Among them, Oligoribonuclease (Orn) is unique as its activity is required for clearing short RNA fragments, which is important for cellular fitness. Here, we show that Orn exhibits exquisite substrate preference for diribonucleotides. While other cellular RNases process oligoribonucleotides down to diribonucleotide entities, Orn is the one and only diribonucleotidase that completes the terminal step of RNA degradation. From this we propose a general model of RNA degradation, wherein a combination of exoribonucleases process oligoribonucleotides down to diribonucleotides and Orn completes RNA recycling by cleaving diribonucleotides to nucleoside monophosphates.

We initially determined the crystal structure of P. aeruginosa Orn (OrnPa) with diribonucleotide substrate; however, crystal packing contacts prevented substrate binding (data not shown). Instead, we were able to crystallize two representative homologs, OrnVc and the human REXO2 (also known as small fragment nuclease or Sfn [Bruni et al., 2013]), bound to the diribonucleotide pGpG (Figure 2—source data 1). Superimposing the two structures indicates their identical fold (rmsd of 0.75 Å for the protomer), which is preserved in the substrate-free Orn structure determined previously (rmsd of 0.54 Å for the protomer). The pGpG-bound structures reveal a narrow active site that is lined by the conserved acidic residues of the signature DEDD motif (D12, E14, and D112 of OrnVc; D15, E17, and D115 of REXO2) and the general base H158 or H162 in OrnVc or REXO2, respectively (Figure 2A and B and Figure 2—figure supplement 1B and Figure 2—source data 2). In OrnVc, the bases of the diribonucleotide buttress against aromatic residues W61 and Y129, the latter being contributed from the second half-side of the dimeric enzyme. Residue L18 in OrnVc (L21 in REXO2) wedges in-between the two bases. Most notably, residues S108, R130, S135 and the hydroxyl group on Y129 (S111, R133, S138, and Y132 in REXO2) form hydrogen bonds with the 5' phosphate of pGpG, capping the substrate. This phosphate cap creates a major constriction of the active site, which is not observed in structurally related 3'−5' exoribonucleases such as RNase T or ExoI (Figure 2C and Figure 2—figure supplement 1 and Figure 2—source data 2). By this assay, quantification of the diffusion zone reveals that OrnVc exhibits the highest affinity for diribonucleotide (Kd pGpG = 90 -/+9 nM), as compared to oligoribonucleotides of greater lengths. Mutations of the central phosphate cap residue R130 to alanine led to complete loss of catalytic activity, comparable to mutants in the DEDD active site motif. While expression of wild-type OrnVc complements the P. aeruginosa ∆orn resulting in a dispersed culture, complementation with variants that carry mutations in either the active site or phosphate cap residues results in cell aggregation indistinguishable from the ∆orn phenotype.

> MSFSDQNLIWIDLEMTGLDPEMHKIIEMATIVTDSELNILAEGPVIAIHQPESELAKMDEWCTTTHTASGLVARVRQSQVSEEEAIDQTLAFLKQWVPEGKSPICGNSIGQDRRFLYKHMPRLEAYFHYRYIDVSTIKELTRRWQPEVLKEFSKTGSHLALDDIRESIAELQFYRKAVFKI>[6x]SNAGWDLTVKMLAGNEFQVSLSSSMSVSELKAQI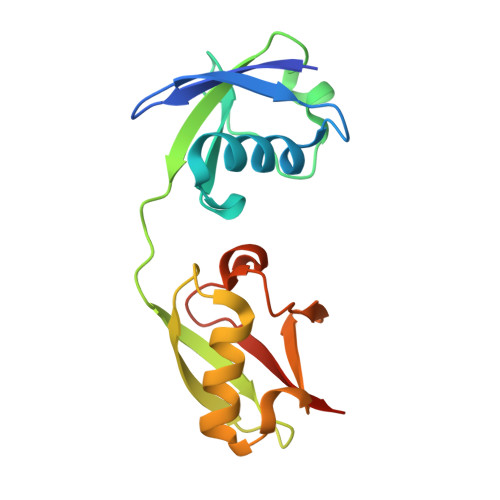TQKIGVHAFQQRLAVHPSGVALQDRVPLASQGLGPGSTVLLVVDKCDEPLSILVRNNKGRSSTYEVRLTQTVAHLKQQVSGLEGVQDDLFWLTFEGKPLEDQLPLGEYGLKPLSTVFMNLRLRGG(3S)-3,4-DI-N-HEXANOYLOXYBUTYL-1-PHOSPHOCHOLINE | C21 H42 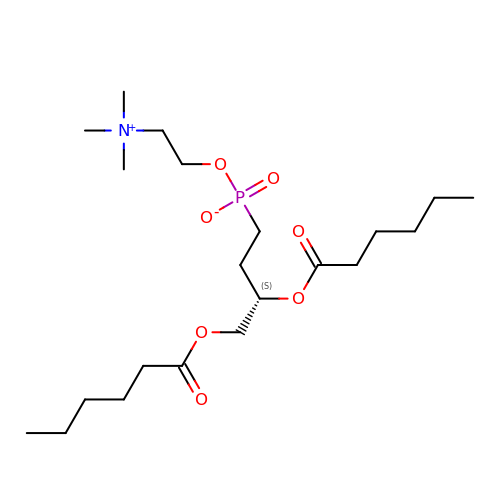N O7 P | BRTDPJPTKQNAET-IBGZPJMESA-N>[6x]MSAHISNVRPDFDREIVDIVDYVMNYEITSKVAYDTAHYCLLDTLGCGLEALEYPACKKLLGPIVPGTVVPNGARVPGTQFQLDPVQAAFNIGAMIRWLDFNDTWLAAEWGHPSDNLGGILATADWLSRNAVAAGKAPLTMKQVLSGMIKAHEIQGCIALENAFNRVGLDHV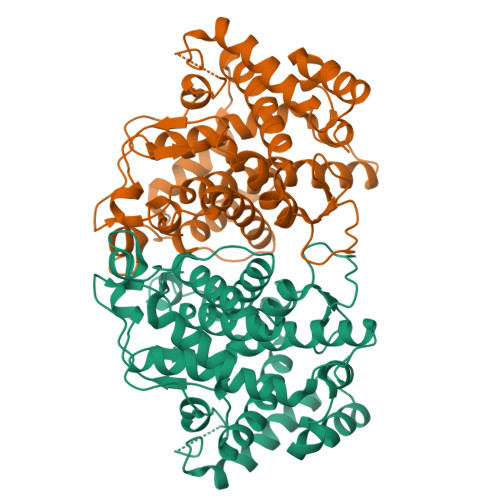LLVKVASTAVVAEMLGLTRDEILNAVSLAWVDGQSLRTYRHAPNTGTRKSWAAGDATSRAVRLALMAKTGEMGYPSALTAKTWGFYDVSFKGETFRFQRPYGSYVMENVLFKISFPAEFHSQTAVEAAMTLYEQMQAAGKTAADIEKVTIRTHEACLRIIDKKGPLNNPADRDHCIQYMVAVPLLFGRLTAADYEDEVAQDKRIDALREKIVCYEDPAFTADYHDPEKRAIGNAISVEFTDGSRFGEVVVEYPIGHARRRADGIPKLIEKFKINLARQFPTRQQQRILDVSLDRARLEQMPVNEYLDLYVI>KESRAKKFQRQHMDSSSSTYCNQMMRRRN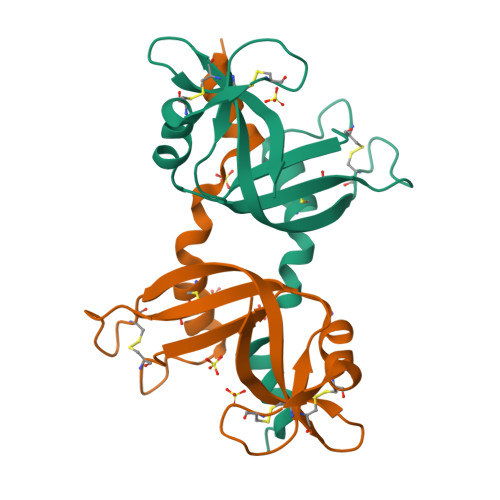MTQGRCKPVNTFVHEPLVDVQNVCFQEKVTCKNGQGNCYKSNSSMHITDCRLTNGSRYPNCAYRTSPKERHIIVACEGSPYVPVHFDASVEDST[4x]>[2x]MRGSHHHHHHGSVLLTMIARVADGLPLAASMQEDEQSGRDLQQYQSQAKQLFRKLNEQSPTRCTLEAGAMTFHYIIEQGVCYLVLCEAAFPKKLAF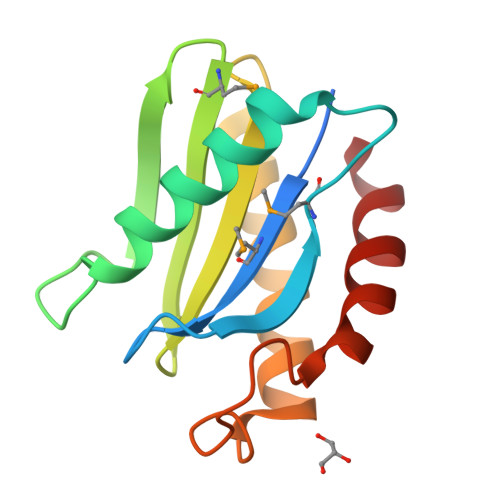AYLEDLHSEFDEQHGKKVPTVSRPYSFIEFDTFIQKTKKLYI> VEATAQETDRPRFSFSIAAREGKARTGTIEMKRGVIRTPAFMPVGTAATVKALKPETVRATGADIILGNTYHLMLRPGAERIAKLGGLHSFMGWDRPILTDSGGFQVMSLSSLTKQSEEGVTFKSHLDGSRHMLSPERSIEIQHLLGSDIVMAFDEVTPYPATPSRAASSMERSMRWAKRSRDAFDSRKEQAENAALFGIQQGSVFENLRQQSADALAEIGFDGYAVGGLAGGEGQDEMFRVLDFSVPMLPDDKPHYLMGVGKPDDIVGAVERGIDMFDCVLPTRSGRNGQAFTWDGPINIRNARFSEDLKPLDSECHCAVCQKWSRAYIHHLIRAGEILGAMLMTEHNIAFYQQLMQKIRDSISEGRFSQFAQDFRARYFARNS

Transfer RNA–guanine transglycosylase (Tgt, EC 2.4.2.29) catalyses the exchange of a specific guanine base in tRNA molecules by a substituted 7-deazaguanine. Bacterial Tgt functions as a homodimer in which the protomer consists of a (βα)8 barrel harbouring a Zn2+ binding subdomain close to the C-terminus. The reaction follows a ping-pong mechanism including a covalent Tgt⋅tRNA intermediate. Hence, in an attempt to generate a model system for the active site of human Tgt and to gain insights into the relevance of particular amino acids for substrate base selectivity, we adapted the Z. mobilis Tgt active site by site-directed mutagenesis in order to mimic that of the human enzyme.

In order to investigate the importance of Gly232 and Val161 in human Tgt for queuine recognition, we created a doubly mutated variant of the Z. mobilis enzyme in which the corresponding Val233 and Cys158 were exchanged by glycine and valine, respectively. Also the electron density maps of the Tgt(Val233Gly)·queuine and Tgt(Cys158Val/Val233Gly)·queuine complex structures enabled reliable placement of the 7-deazaguanine scaffold of the ligand which is, in both cases, similarly bound as in the Tgt(Cys158Val)·queuine complex. In both maps fragmentary density is visible for the dihydroxy-cyclopentenyl substituent (7H as well as 8F, 8H). Figures 7F and 7H show that the mutation of Val233 to glycine results in a considerable gain of space in the substrate binding pocket which allows the dihydroxy-cyclopentenyl of queuine to occupy the cavity located between Gly233 and the side chain of Cys/Val158. Within this cavity the dihydroxy-cyclopentenyl apparently has no specific interaction with the protein. As a consequence, it seems to be highly flexible which is reflected by the ill-defined electron density assigned to this moiety in both structures. As in the structure of queuine-bound Tgt(Cys158Val), nearly no electron density can be attributed to the side chain of Val158 in the Tgt(Cys158Val/Val233Gly)·queuine complex structure, indicating an increased mobility of this residue upon the binding of queuine. Also, in agreement with the structure of queuine-bound Tgt(Cys158Val), the positioning of the Val158 main chain atoms suggests a shift of this residue towards the ligand which is not concomitant with a rotation of the Thr159 side chain. The crystal structures of Tgt(Val233Gly) and Tgt(Cys158Val/Val233Gly) with queuine reveal that the Val233Gly exchange allows the dihydroxy-cyclopentenyl substituent to occupy the created cavity between position 233 and 158. The adopted binding mode of queuine will not interfere sterically with the sugar-phosphate backbone of bound tRNA. Solely in the case of Tgt(Cys158Val/Val233Gly), the variant that should best approach the eucaryotic enzyme, the result of the trapping experiment indicates that the covalent enzyme·tRNA complex may, though to a low extent, be able to bind queuine.> GPHMLEAEHPLQYNYTFWYSRRTPGRPTSSQSYEQNIKQIGTF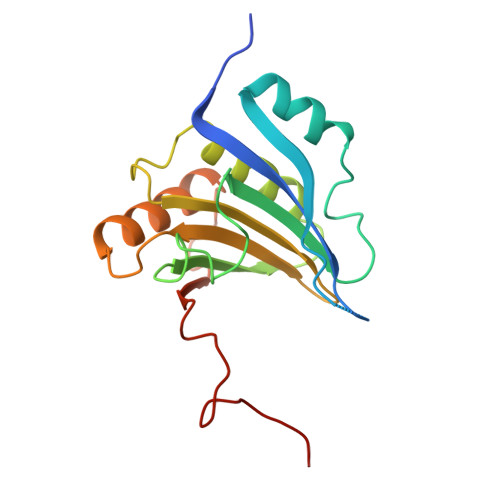ASVEQFWRFYSHMVRPGDLTGHSDFHLFKEGIKPMWEDDANKNGGKWIIRLRKGLASRCWENLILAMLGEQFMVGEEICGAVVSVRFQEDIISIWNKTASDQATTARIRDTLRRVLNLPPNTIMEYKTHTDSIKMPGRLGPQRLLF> GSPSTCTVTIEVLGHELDFAQDPNSKHLGTTVWDAS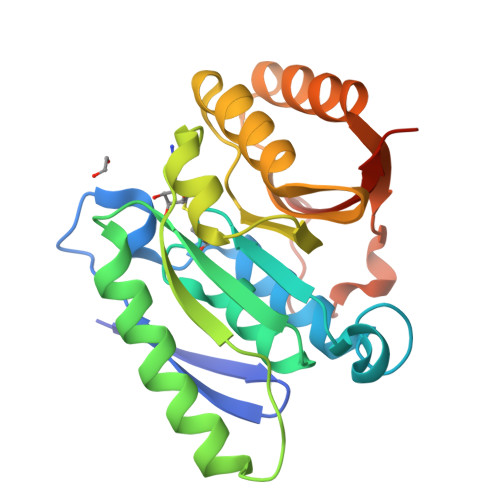MVFAKYLGKNSRKGRFSSSKLKGKRAIELGAGCGVAGFALAMLGCDVVTTDQKEVLPLLKRNVEWNTSRIVQMNPGSAFGSLRVAELDWGNEDHITAVEPPFDYVIGTDVVYSEQLLEPLLRTILALSGPKTTVMLGYEIRSTVVHEKMLQMWKDNFEVKTIPRSKMDGEYQDPSIHLYIMAQKSAAESSAAA> MATLLRSLALFKRNKDKPPITSGSGGAIRGIKHIIIVPIPGDSSITTRSRLLDRLVRLIGNPDVSGPKLTGALIGILSLFVESPGQLIQRITDDPDVSIRLLEVVQSDQSQSGLTFASRGTN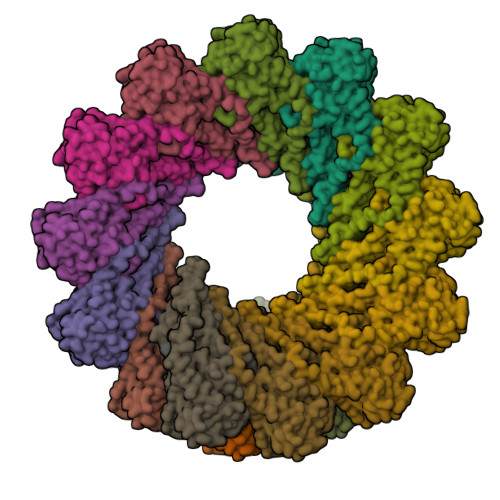MEDEADQYFSHDDPISSDQSRFGWFENKEISDIEVQDPEGFNMILGTILAQIWVLLAKAVTAPDTAADSELRRWIKYTQQRRVVGEFRLERKWLDVVRNRIAEDLSLRRFMVALILDIKRTPGNKPRIAEMICDIDTYIVEAGLASFILTIKFGIETMYPALGLHEFAGELSTLESLMNLYQQMGETAPYMVILENSIQNKFSAGSYPLLWSYAMGVGVELENSMGGLNFGRSYFDPAYFRLGQEMVRRSAGKVSSTLASELGITAEDARLVSEIAMHTTEDKVEHHHHHHHH>SNAMKKLAISIGDINSIGLEILVRSHEELSKICTPFYFIHESLLNKALKLLNLKLFNAKIVAFKDDKDYEFNFIKKENSLEIYSFCLPLGFKVDENFEIQAGEIDAKSGLYGFLSFKAASYFVYEKHAHALLTLPIHKKAWEDAGLKYKG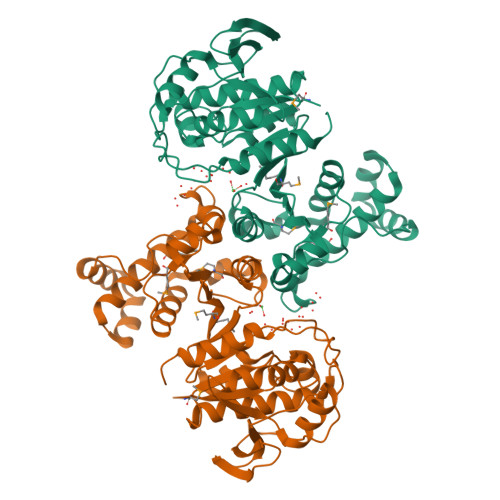HTDALRDFFKKNAIMMLGCKELFVGLFSEHIPLAKVSKKITFKNLSIFLKDFYKETHFKKMGLLGFNPHAGDYGVIGGEEEKIMEKAIAFVNAFLHSKKDEKFFKKALKDENLQKELLLNFKGKGVYLPYPLVADTAFTKTGLKNCNRLVAMYHDLALAPLKALYFDKSINVSLNLPIIRVSVDHGTAFDKAYKNAKINTKSYFEAAKFAINLHSKA[4x]> GSGRGLGPLQIWQTDFTLEPRMAPRSWLAVTVDTASSAIVVTQHGRVTSVAAQHHWATAIAVLGRPKAIKTDNGSCFTSKSTREWLARWGIAHTTGIPGNSQGQAMVERANRLLKDKIRVLAEGDGFMKRIPTSKQGELLAKAMYALNHF

During the replicative cycle of retroviruses, the retrotranscribed viral DNA is integrated into the host chromosome by the viral integrase protein (IN). Retroviral IN consists of three domains: the zinc-binding N-terminal domain (NTD), the catalytic core domain (CCD) and the C-terminal domain (CTD). The central CCD contains an invariant D,D(35)E motif, which forms a catalytic triad with two sites that can coordinate various divalent cations (Mg(II), Mn(II), Zn(II), Cd(II), Ca(II)) although Mg(II) is the likely metal cofactor in vivo. Rous-associated virus type 1 (RAV-1) is a replication-competent alpharetrovirus, member of ASLV subgroup A; the INs of this retrovirus genus are a good model for HIV IN [28].

As a control, the A182T mutant of RAV-1 IN CCD (termed RAV-1 IN CCDA182T), corresponding to the RSV-A IN CCD sequence, was purified and the crystallization conditions for both RAV-1 IN CCD and RSV-A IN CCD were tested; that is, a MES buffer at pH 6.0 and a citrate buffer at pH 6.2, respectively. Large crystals were obtained with the second set of conditions. Further, the huge crystals of RAV-1 IN CCDA182T were isomorphous to those of RSV-A IN CCD obtained under the same conditions. They belonged to space group P43212 with one molecule in the asymmetric unit. Synchrotron data for these crystals were collected to 1.55 Å resolutions. The refined structure of RAV-1 IN CCDA182T contains 137 residues, 1 citrate molecule and 122 water molecules (right). The 145–152 loop is disordered and is not observed in the electron density map, as in RSV-A IN CCD. Thus, the tertiary structure of RAV-1 IN CCD is nearly identical to that of RSV-A IN CCD, equivalent to that of RAV-1 IN CCDA182T (r.m.s. deviation of 0.4 Å on 132 Cα pairs) and respects the ribonuclease H fold. The A182T substitution mostly affects the side-chain orientation of the neighboring Arg179 of the α4-α5 loop. This arginine is hydrogen bonded to the side-chain oxygen atom OG of Thr182 in RSV-A IN CCD, whereas a similar contact is impossible with the aliphatic Ala182 in RAV-1 IN CCD. Thus, the A182T substitution influences crystal assembly via Arg179 and, either large tetragonal crystals or tiny hexagonal microcrystals are observed for RAV-1 IN CCDA182T, whereas only hexagonal crystals are obtained for RAV-1 IN CCD.> GPT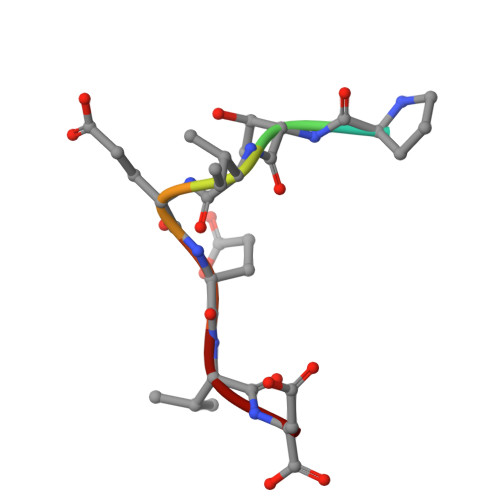IEEVD>MQKQVKISGKSKENMSLLKHLKGDVQGKELVIEDSIVNERWKQVLKEKIDIEHDLFNYQKNREISKVPFLPVDRLITNDEVEDILNTLTEVLPTGKFTSGPYLEQFEKVLSTYLHKRYVIATSSGTDAIMIGLLALGLNPGDEVIMPANSFSATENAVLASGGVPIYVDINPQTFCIDPDKIEEAITPYTKFILPVHLYGKHSDMQHIRQIANRYKLKVIEDACQGIGLTDLGKYADITTLSFNPYKNFGVCGKAGAIATDNEELAKKCIQFSYHGFEVNVKNKKVINFGFNSKMDNLQAAIGLERMKYLSLNNFKRLF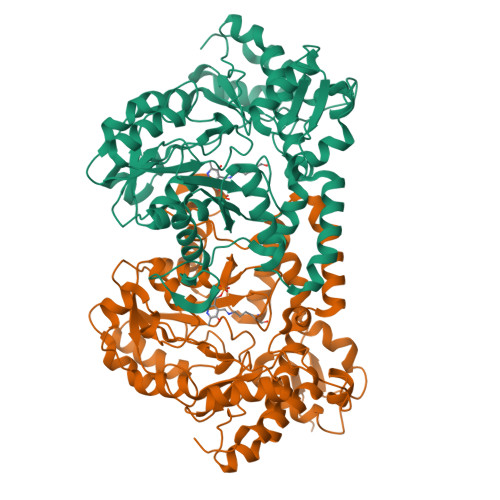LADRYITQLAELQNKGYIELPELSEDHVWHLFPIKVRTEDRADIMTKLNEDFGVQTDVYYPILSHMQKTPLVQDKYAGLQLVHTEKAHSQVLHLPLYPSFTLEEQDRVMEGLFHVIKQEIGV[2x]>[2x]GHMVSRIEQRLIDKGLKVTDQRRVIAQVLSDSADHPDVEEVYRRATAKDPRISIATVYRTVRLFEEESILERHDFGDGRARYEEAPSEHHDHLIDVNSARVIEFTSPEIEAL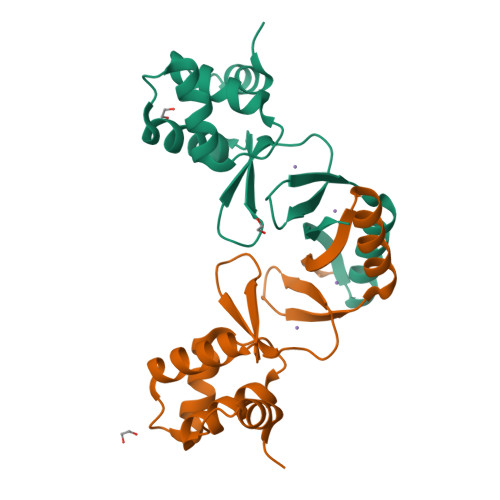QREIARKHGFRLVGHRLELYGVPLTSGGDSDDK>[4x]MPPNLTGYYRFVSQKNMEDYLQALNISLAVRKIALLLKPDKEIEHQGNHMTVRTLSTFRNYTVQFDVGVEFEEDLRSVDGRKCQTIVTWEEEHLV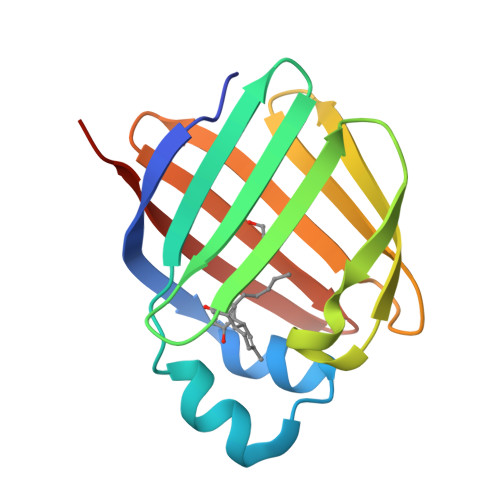CVQKGEVPNRGWRHWLEGEMLYLELTARDAVCEQVFRKVRLVPR> GPHMADLF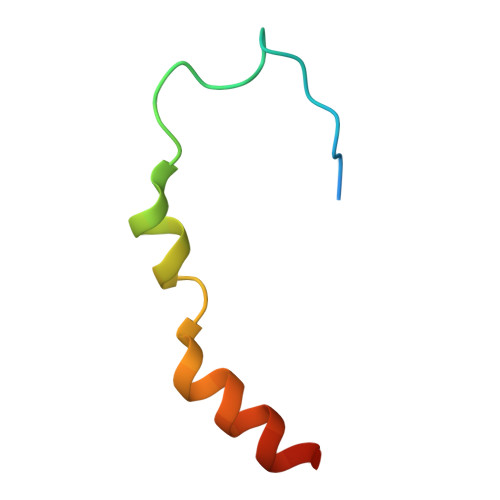GDDIEEIPDTDFDFEGNLALFDKAAVFEEIDTYERR The T4BS secretion coupling complex of L. pneumophila comprises the inner membrane AAA+ ATPase DotL (IcmO) and two inner membrane/cytoplasmic components, DotM (IcmP) and DotN (IcmJ). In this study, we determine the crystal structure of the cytoplasmic domain of DotM and observe large patches of basic residues, leading us to hypothesize that DotM might form the recruiting platform for Glu-rich motif-containing effectors. Our results suggest that DotM’s cytoplasmic domain is capable of binding directly another subgroup of Legionella effectors that contain acidic Glu-rich motifs at their C terminus.

Further binding studies were conducted with several DotM mutants, where Arg residues (single or double) on the protein’s surface were mutated to Glu. Five mutants were produced: R196E/R197E (termed “M1”), R314E/R315E (termed “M2”), R347E/R348E (termed “M3”), R217E (termed “M4”), and R262E (termed “M5”). Binding was abrogated in M1, M2, and M4, indicating that these Arg patches are involved in binding of acidic Glu-rich peptides. M3 and M5 were unaffected suggesting that they are not involved in Glu-rich sequence binding. The Lpg1663 and the consensus OSM peptide was also assessed for binding to the M1 and M2 mutants and binding was found to be also abrogated (Fig. 4 and Table 3; Lpg1663- or OSM-binding to other mutants was not tested because wild-type DotM, M1 and M2 display the same binding behavior for the Lpg1663 and OSM peptides as for CegC3). To ascertain that the observed binding deficiency in M1, M2, and M4 variant proteins was not due to folding defects caused by the mutations, these three proteins were crystallized and their structures were determined and shown to be virtually identical to the wild-type protein. Thus, the mutations do not introduce structural defects, suggesting that the ITC binding results reflect an effective role of the residues in binding. The final model suggests that CegC3 is primarily helical. Binding is observed between the main middle Glu-rich helical motif of CegC3 (residues E155, E158, and E159; see numbering in Table 2 and interactions in Fig. 5) to the “central patch” residues R314 and R315, as well as between R217 of DotM to peptide residue E162. Two were successfully obtained (M1 and M4) but attempts at introducing M2 failed for reasons that remain unclear but could be due to a destablization of the DotMLN coupling complex resulting in activation of processes that are stressful to the cell. Intriguingly, among the residues we show here to be involved in this recognition process, only R314 is highly conserved, whereas residues R196, R197, and R217, despite their importance in Glu-rich peptide binding, exhibit a lower conservation.

>GPSGGGADVNKGPWAMALTPMEFARKYNLLRKDDALLDNPVPGEEMTAGIRRGDAKRVFTMQLGPYWDGFERCSPQAYALSAVFMARMNRDRDAANNILKVLDKTFVDGKPDFSVARPVMKKYQNSELVQEVVAKHAYVLTVIASLLEAAREDGVVPSSEFLWLKPVDEELWYMLNCVGRQTPYSEVAGPFAHWKAEKEMGRRSLVPMIDEAIRALEIAVKEVRLTPRQMEELEP[2x]7-methoxy-6-methylpteridine-2,4-diamine 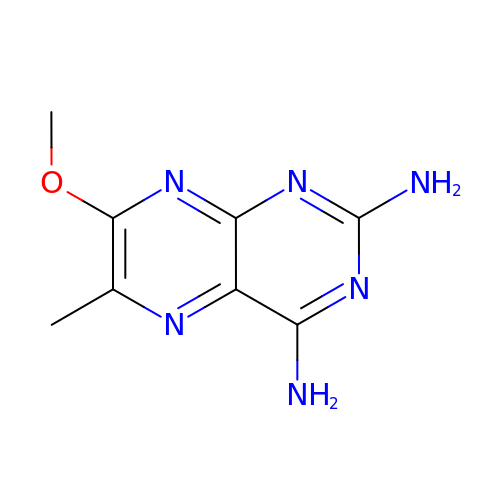| C8 H10 N6 O | PBUUVJRZGWWXQU-UHFFFAOYSA-N>MGHHHHHHHHHHSSGHIEGRHMMRAIWTGSIAFGLVNVPVKVYSATADHDIRFHQVHAKDNGRIRYKRVCEACGEVVDYRDLARAYESGDGQMVAITDDDIASLPEERSREIEVLEFVPAADVDPMMFDRSYFLEPDSKSSKSYVLLAKTLAETDRMAIVHFTLRNKTRLAALRVKDFGKREVMMVHTLLWPDEIRDPDFPVLDQKVEIKPAELKMAGQVVDSMADDFNPDRYHDTYQEQLQELIDTKLEGGQAFTAEDQPRLLDEPEDVSDLL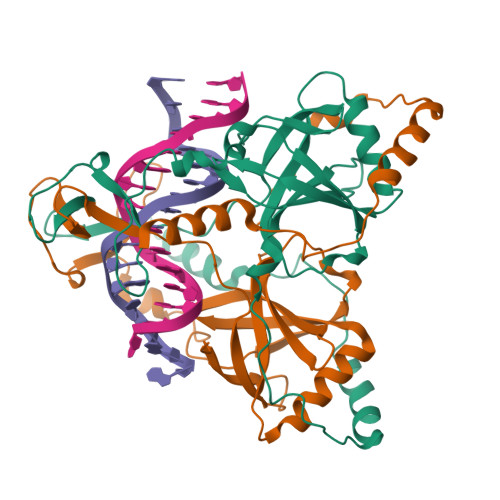AKLEASVKARSKANSNVPTPP[2x]>MDYKDDDDKGSSSSNVEVFIPVSQGNTNGFPATASNDLKAFTEGAVLSFHNICYRVKLKSGFLPCRKPVEKEILSNINGIMKPGLNAILGPTGGGKSSLLDVLAARKDPSGLSGDVLINGAPRPANFKCNSGYVVQDDVVMGTLTVRENLQFSAALRLATTMTNHEKNERINRVIQELGLDKVADSKVGTQFIRGVSGGERKRTSIGMELITDPSILFLDEPTTGLDSSTANAVLLLLKRMSK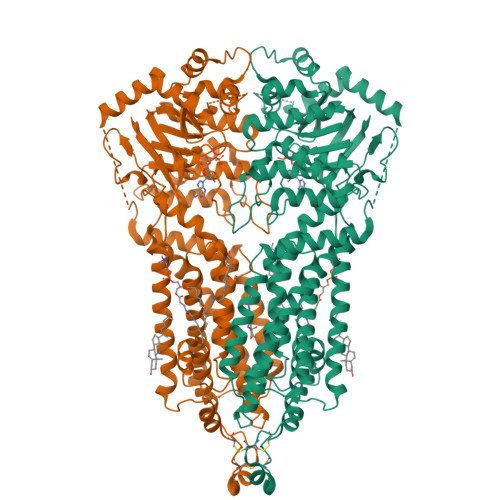QGRTIIFSIHQPRYSIFKLFDSLTLLASGRLMFHGPAQEALGYFESAGYHCEAYNNPADFFLDIINGDSTAVALNREEDFKATEIIEPSKQDKPLIEKLAEIYVNSSFYKETKAELHQLSGGEKKKKITVFKEISYTTSFCHQLRWVSKRSFKNLLGNPQASIAQIIVTVVLGLVIGAIYFGLKNDSTGIQNRAGVLFFLTTNQCFSSVSAVELFVVEKKLFIHEYISGYYRVSSYFLGKLLSDLLPMRMLPSIIFTCIVYFMLGLKPKADAFFVMMFTLMMVAYSASSMALAIAAGQSVVSVATLLMTICFVFMMIFSGLLVNLTTIASWLSWLQYFSIPRYGFTALQHNEFLGQNFCPGLNATGNNPCNYATCTGEEYLVKQGIDLSPWGLWKNHVALACMIVIFLTIAYLKLLFLKKYS[2x]Recent work has revealed that Mmi1 interacts with Erh1 to form a complex, called EMC14, and loss of Mmi1 affects recruitment of Erh1 and its associated RNA processing activities to target transcripts. Here, we present the co-crystal structure of Erh1 in complex with the amino-terminal domain of Mmi1. Our structure reveals that Mmi1 binds homodimers of Erh1 in a 2:2 stoichiometry, via a conserved molecular interface characteristic of ERH family proteins. Structure-guided mutational analysis shows that the Mmi1-Erh1 interaction is essential for facultative heterochromatin assembly and for silencing of gametogenic genes.

We used a (Gly-Ser-Ser)5 linker to fuse Erh1 and Mmi195–122 in tandem. The co-crystal structure was resolved to 2.7 Å resolution by molecular replacement. Consistent with the 2:2 stoichiometry model based on the results from the SEC experiments, the co-crystal structure revealed that Erh1 forms a homodimer, with two Mmi1 subunits bound on the surface of the Erh1 homodimer. Overall, the Erh1 monomer adopted a typical ERH fold, characterized by a four-stranded antiparallel β-sheet (β1–β4) and three α-helixes (α1–α3), with the α-helixes on one face of the sheet. The outside faces of the β-sheets of two monomers constituted the homodimer interface and formed a pseudo-β-barrel, burying about 1000 Å2 of solvent-exposed area. Each Mmi1 peptide was bound across the β2 edge of the β-sheet of each Erh1 monomer, with the amino-terminal residues (Mmi1Lys96-Mmi1Cys103) located in the groove between α-helix α1 and the β-sheet, whereas the carboxy-terminal residues (Mmi1Thr104-Mmi1Arg119) were bound to the hydrophobic core of the dimer pseudo-β-barrel. When bound to Erh1, the carboxy-terminal residues of the Mmi195–122 peptide (109SYEWPYFRSLR119) folded into two consecutive helices, consisting of a 310 helix (H1) and an α-helix (H2). The Mmi1Trp112 aromatic ring stretched into a deep hydrophobic pocket formed by Erh1His9, Erh1Val70, Erh1Ile11, Erh1Leu13, and Erh1Trp25, with its Nε nitrogen forming a hydrogen bond with the side chain of Erh1Asp27. Indeed, Mmi1Trp112 is crucial for EMC formation as substitution with alanine disrupted Mmi1-Erh1 interaction as confirmed by GST pull-down assay and ITC. We also observed that the H1 helix toward the amino-terminus, Mmi1 (96KYDFSRHCTDYGH108), adopted a long structural loop conformation featuring several turns, which was constrained by an intertwined network of both intra- and inter-molecular interactions.

>[2x]MGHHHHHHMSPPPAESHIILLIQQGSDPKTRIWSDHCSLRSAIEYIVGVYQTNQAVSEKESIDVSRFFNFFDEIYDCVPLVYDRHFRAYIPHEKQWLLHHAQEYLTAARQIPGSSGSSGSSGSSGSSGKYDFSRHCTDYGHSYEWPYFRSLRRES>MSHPPSNTPPVKPGGLPLLGHILEFGKNPHAFLMALRHEFGDVAEFRMFHQRMVLLTGSQASEAFYRAPDEVLDQGPAYRIMTPIFGRGVVFDARIERKNQQLQMLMPALRDKPMRTYSEIIVAEVEAMLRDWKDAGTIDLLELTKELTIYTSSHCLLGAEFRHELNTEFAGIYRDLEMGIQPIAYVFPNLPLPVFKRRDQARVRLQELVTQIMERRARSQERSTNVFQMLIDASYDDGSKLTPHEITGMLIATIFAGHHTSSGTTAWVLIELLRRPEYLRRVRAEIDALFETHGRVTFESLRQMPQLENVIKEVLRLHPPLILLMRKVMKDFEVQGMRIEAGKFVCAAPSVTHRIPELFPNPELFDPDRYTPERAEDKDLYGWQAFGGGRHKCSGNAFAMFQIKAIVCVLLRNYEFELAAAPESYRDDYRKMVVEPASPCLIRYRRRDAPAAVDAKASAGEAPAETLRGAFRVTVDRDLCKGHGNCMAE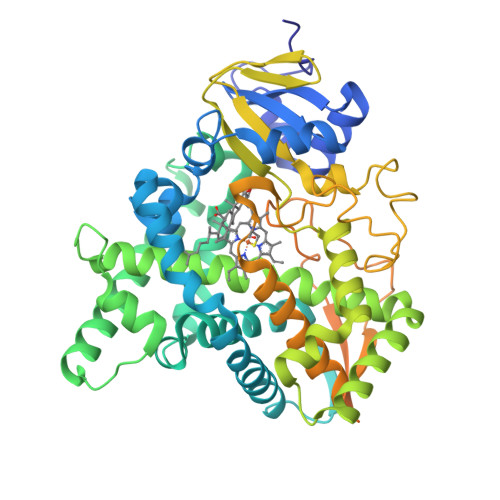APEIFRVDEDGRLTLLSETPDPVLVGAALAAERFCPARAIKILPQRDPATRDRSLSPSGED[4x]>MASGCSTVDTVKDFNKDNFFTGSWYITHYKLGDSTLEVGDKNCTKFLHQKTADGKIKEVFSNYNPNAKTYSYDISFAKVSDFDGNNGKYTAKNVIVEKDGRKIDERTLQVSYIDTDYSKYSVVHVCDPAA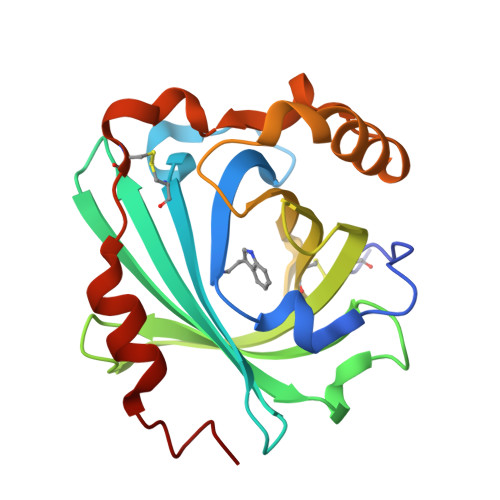PDYYLYAVQSRTENVKEDVKSKVEAALGKVGLKLSGLFDATTLGNKCQYDDETLQKLLKQSFPNYEK[4x]[(2~{R},3~{S},4~{S},5~{R})-3,4-bis(oxidanyl)-5-[3-(4-phenyl-1,2,3-triazol-1-yl)propyl]oxan-2-yl]methyl 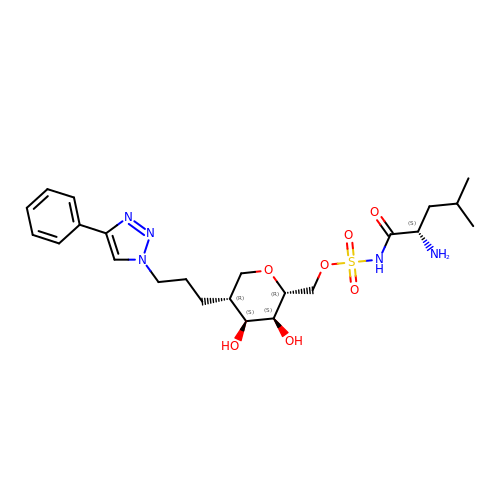~{N}-[(2~{S})-2-azanyl-4-methyl-pentanoyl]sulfamate | C23 H35 N5 O7 S | GZWHBJQJDPZTNY-WQIFRTTPSA-N> MTSIKPFQMEDLFELNPVNLDPLTENFNVSFYSQYLIEWPQLFYKSVETPNGQASGYMMAKTEGQLSKKEWHTHITAVTVLDQYRRIGLASKLCLELENLTQVKDTLFIDLFV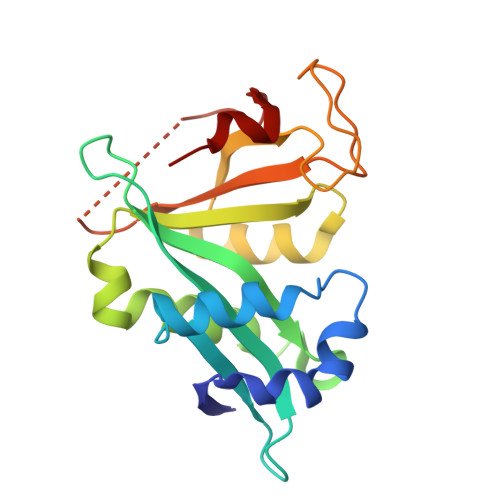KVTNTLGRILYEKLGYSVFRRVVGYYGREIQKDRNKIDDSVDAFDMRKLLPRDVNNETVRENGEKVYVLPNEIVF(2Z,4E)-5-carbamimidamido-2-iminopent-4-enoic acid | C6 H10 N4 O2 | 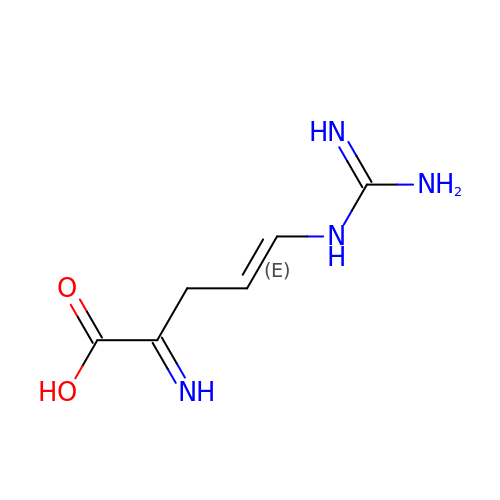DTYASQOTNAATQJ-QJBDDWKRSA-N 (4S,4aS,6aR,8R,9R,11E,12aR,14aS,17E,18aR,18bR)-9-ethyl-4,8,19-trihydroxy-11,12a,13,18a-tetramethyl-2,3,4,4a,6a,7,8,9,10,12a,13,14,18a,18b-tetradecahydro-14a,17-(metheno)cyclobuta[b]naphtho[2,1-j][1]azacyclotetradecine-16,18(1H,15H)-dione 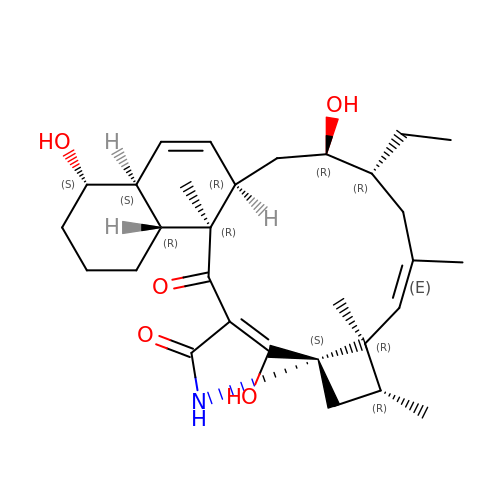| C30 H43 N O5 | FPGYXUMODXYNNS-BKXSIXICSA-N> MTQEFIDKVSSYLTPDVDIAPISQGAEAIVFTTTTHPYLPRAKDSHQKYIIKYRPPKRYRHPQIDQALTKHRTLNESRLLAKLYLIPGLCVPQLIAC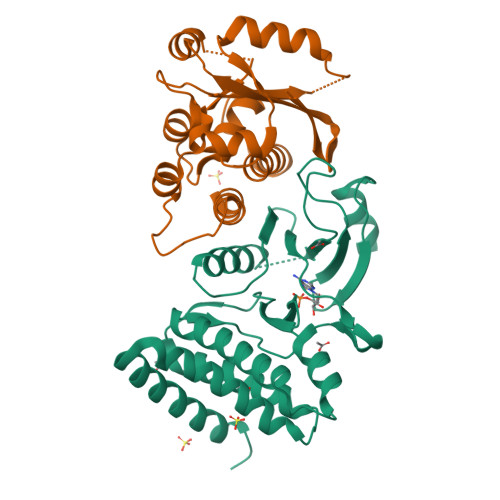DPYNGFIWLEFLGEDLPGGHGFSNLKNFLWMHDQDPYSDLVATTLRKVGRQIGLLHWNDYCHGDLTSSNIVLVRDGARWTPHLIDFGLGSVSNLVEDKGVDLYVLERAILSTHSKHAEKYNAWIMEGFEEVYREQGAKGAKKLKEVTKRFEEVRLRGRKRSMLG;> MVVSIIPQFPDIKVSLALFEQVKNAKEIRSKMSELSTSFAFIDPRLVCSGEQMYSAIYKTLIEVKYNKMRTRNLNSECVLCLSPTSNISDAFLKFGIKDDSSQLICLKFHTNTDDVDKEQLRTIMTSIVKGQEIEFNDDNLSRFYDEALIRKIYKLSDDFKPQDVNGLSRALVDAIQLRGVHHHHHH> DQHKAHKAILAYEKGWLAFSLAMLFVFIALIAYTLATHTAGVIPAGKLERVDPTTVRQEGPWADPAQAVVQTGPNQYTVYVLAFAFGYQPNPIEVPQGAEIVFKITSPDVIHGFHV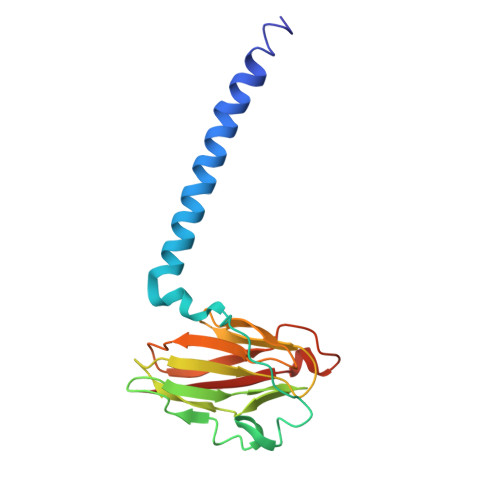EGTNINVEVLPGEVSTVRYTFKRPGEYRIICNQYCGLGHQNMFGTIVVKE> MLPGTFFEVLKNEGVVAIATQGEDGPHLVNTYNSYLKVLDGNRIVVPVGGMHKTEANVARDERVLMTLGSRKVAGRNGPGT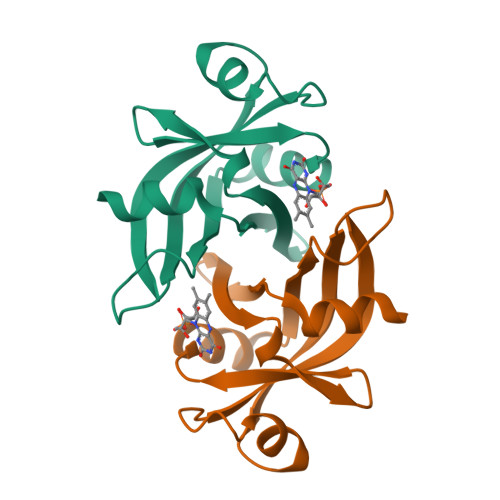GFLIRGSAAFRTDGPEFEAIARFKWARAALVITVVSAEQTL During virus assembly, a primary role of the MA domain is to bring Gag to the inner leaflet (IL) of the plasma membrane via its covalently attached N-terminal myristate group and highly basic region (HBR). The MA HBR promotes Gag membrane binding by engaging in electrostatic interactions with the IL of the plasma membrane. The HIV-1 MA protein forms trimers that assemble into a hexameric lattice with central cavities at points of sixfold symmetry on PS- and PI(4,5)P2-enriched membranes. During HIV-1 maturation, the MA lattice undergoes structural rearrangement, with mature virions displaying a more regular hexameric lattice and smaller central hexameric apertures compared to their immature counterparts.

Here, we examine maturation of an MA triple mutant, L20K/E73K/A82T, which, despite replicating similarly to wild-type (WT) in some cell lines, exhibits distinct biochemical behaviors that suggest altered MA-MA interactions. Cryo–electron tomography with subtomogram averaging reveals that, although the MA lattice in immature L20K/E73K/A82T virions closely resembles that of the WT, mature L20K/E73K/A82T virions lack a detectable MA lattice. In addition to the significant density loss in the center of the L20K/E73K/A82T MA trimer, there was an unpaired density gain at the C terminus of L20K/E73K/A82T MA pointing to the CA layer (blue arrow), suggesting that this region is likely less flexible than the WT counterpart. Additionally, the electrostatic potential on the surface of MA facing the membrane is also more positive than the WT, due to the L/K and E/K changes in the L20K/E73K/A82T mutant. But more intriguingly, in L20K/E73K/A82T mutant VLPs, the intersection points became concentrated at the threefold axis, and the registration between the MA trimer and the CA trimer is much stronger than WT. This is consistent with the observation of a more ordered MA C terminus in the L20K/E73K/A82T mutant MA compared to the WT. In the L20K/E73K/A82T mutant MA, however, E73 is substituted with K73, which forms salt-bridges with E39 and E41 and transiently with other lipid headgroups but does not contribute to Na+ ion coordination. As a result, interactions at the trimer centers in mutant MA are only mediated by salt bridges with R42, making them less stable compared to WT MA. In the immature L20K/E73K/A82T mutant, the absence of central density, coupled with upward reorientation of R42 in the AlphaFold2 prediction, as well as the E73K mutation, is presumed to enhance interactions with lipid headgroups, consistent with the role of R42 in phospholipid binding. The collective structural modifications induced by L20K and E73K and the repositioning of R42 create a highly positive surface for phospholipid binding and docking, offering an explanation for the increased Gag binding affinity observed for the L20K/E73K/A82T mutant.

>[39x]GARASVLSGGELDKWEKIRKRPGGKKQYKLKHIVWASRELERFAVNPGLLETSEGCRQILGQLQPSLQTGSEKLRSLYNTITVLYCVHQRIDVKDTKEALDKIEEEQNKSKKKAQ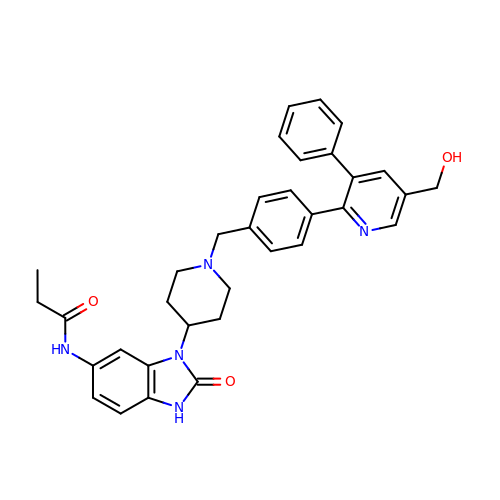~{N}-[3-[1-[[4-[5-(hydroxymethyl)-3-phenyl-pyridin-2-yl]phenyl]methyl]piperidin-4-yl]-2-oxidanylidene-1~{H}-benzimidazol-5-yl]propanamide | C34 H35 N5 O3 | XYDKMXKWNYYJAT-UHFFFAOYSA-N>GPLGSMFSRIRLATPSDVPFIHKLIHQMAVFERLTHLFSATESGLASTLFTSRPFQSFTVFLLEVSRSPFPATITSSPSPDFTPFFKTHNLDLPIDDPESYNFSPDMLNDVVVAGFVLFFPNYSSFLSKPGFYIEDIFVREPYRRKGFGSMLLTAVAKQAVKMGYGRVEWVVLDWNVNAIKFYE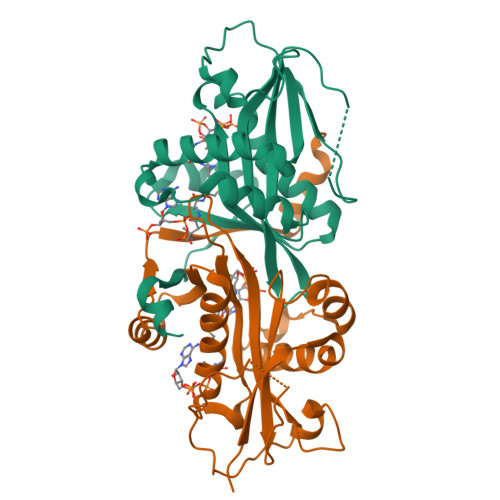QMGAQILQEWRVCRLTGDALEAFDQVNI[2x]> MTTVLVTGGAGFIATHTDIELLNKGYDVISVDNYGNSSPVALERVEQITGKPVKRYDGDVRDEALMERVFAENNIDWVIHFAGLKAVGESVAKPIEYYDNNLYSTLVLLKVMKKHNVKKIIFSSSATVYGTPKELPITEETPTGGTTNPYGTSKLFQEQILRDVHVADPSWTIVLLRYFNPVGAHESGLLGEDPKGIPANLTPYVAKVAVGELKEVQVYGDDYDTPDGTGVRDYIHVVDLAKGHVAVIDHIDKEGVFVYNLGTGHGYSVLEVIKAYEKAAGHPIPYAIKPRRPGDIAACYADASKAEKELGWKAELTIDDMAASSLNWQTKNPNGFRDAE

GalE catalyzes NAD+-dependent oxidoreductive interconversion of gluco- and galacto-hexoses (C4-epimerization) linked to UDP and generally plays a key role in the metabolism of galactose in various organisms. Group 1 enzymes are further divided into two subfamilies (1a and 1b) due to their separation in the phylogenetic tree. bGalE catalyzes epimerization reactions of UDP-Gal into UDP-Glc and UDP-GalNAc into UDP-GlcNAc with the same level of activity and is categorized into group 215. The dimer interface consists of a bundle of 4 α-helices and contains 8 hydrogen bonds and 4 salt bridges. bGalE has a typical fold of SDR superfamily. The overall monomer protein structure can be roughly divided into an N-terminal NAD+ binding domain (N domain, residues 1–177 and 236–262) and a C-terminal UDP-sugar binding domain (C domain, residues 178–235 and 263–340).

Since the recombinant bGalE protein contains one NAD+ molecule per monomer as a noncovalently bound prosthetic group, we prepared ternary complex form crystals with UDP, UDP-Glc, or UDP-GlcNAc by cocrystallization and determined their crystal structures at 1.8–2.0 Å resolution. The electron densities of UDP, UDP-Glc, and UDP-GlcNAc were clearly observed. In bGalE, the UDP moiety is recognized by stacking and hydrophobic interactions by Tyr291 and Leu201, hydrogen bonds by Asp295 and Asn180, and salt bridges by Arg292 and Arg232. The hydroxy groups of the Glc moiety are recognized by hydrogen bonds from the main chain of Lys85 (O2 and O3) and the side chain atoms of Asn200 (O2), Tyr150 (O3 and O4), Ser125 (O4), and Asn180 (O6). In the UDP-GlcNAc complex, the side chain of Asn200 adopts a distinct conformation (designated as “swing out”) from that in the UDP-Glc complex (“swing in”) to accommodate the 2-N-acetyl group. The glucopyranose rings of the UDP-sugars in bGalE are both in the “standard” conformation, in which the H4 atom faces the pro-S side of the NAD+ nicotinamide. The distances between the C4 atom of the sugar ring and the C4 atom of the nicotinamide ring are 3.4 Å and 3.5 Å in the UDP-Glc and UDP-GlcNAc complex structures, respectively. Tyr150 forms a direct hydrogen bond (2.6 Å) with the O4 atom in both the UDP-Glc and UDP-GlcNAc complex structures. Lys154 contributes to the binding of nicotinamide ribose, while Ser125 and Tyr150 form direct hydrogen bonds with the O3 and O4 hydroxy groups of the Glc or GlcNAc, respectively.>[4x]SQTVHFQGNPVTVANS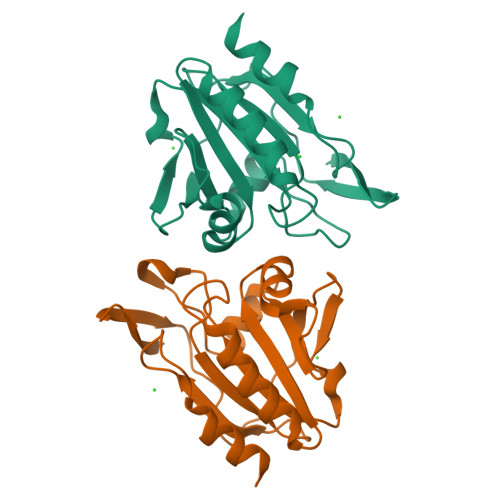IPQAGSKAQTFTLVAKDLSDVTLGQFAGKRKVLNIFPSIDTGVCAASVRKFNQLATEIDNTVVLSISADLPFAQSRFSGAEGLNNVITLSTFRNAEFLQAYGVAIADGPLKGLAARAVVVIDENDNVIFSQLVDEITTEPDYEAALAVLKA>TAGGGTT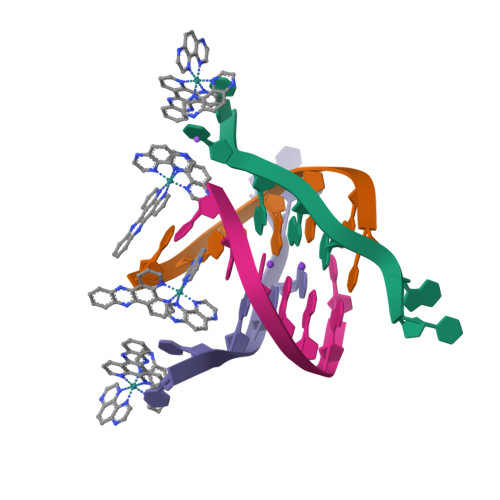[4x]>[2x]GPVAVTLHNEAITYTADITVGSDNQKLNVIVDTGSSDLWIPDSNVICIPKWRGDKGDFCKSAGSYSPASSRTSQNLNTRFDIKYGDGSYAKGKLYKDTVGIGGVSVRDQLFANVWSTSARKGILGIGFQSGEATEFDYDNLPISLRNQGIIGKAAYSLYLNSAEASTGQIIFGGIDKAKYSGSLVDLPITSEKKLTVGLRSV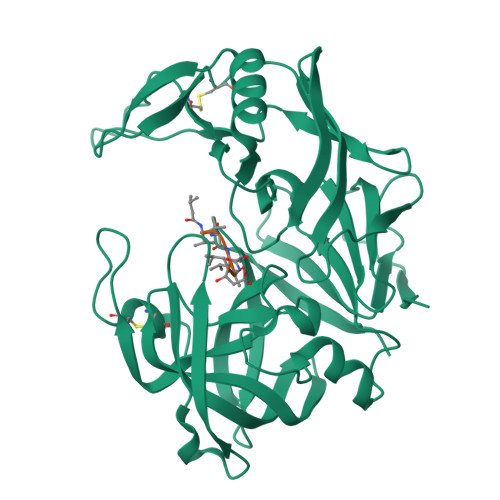NVRGRNVDANTNVLLDSGTTISYFTRSIVRNILYAIGAQMKFDSAGNKVYVADCKTSGTIDFQFGNNLKISVPVSEFLFQTYYTSGKPFPKCEVRIRESEDNILGDNFLRSAYVVYNLDDKKISMAPVKYTSESDIVAIN>[2x]SMPITPQQALQRTIEHREIFHDEMVDLMRQIMRGEVSDAMVS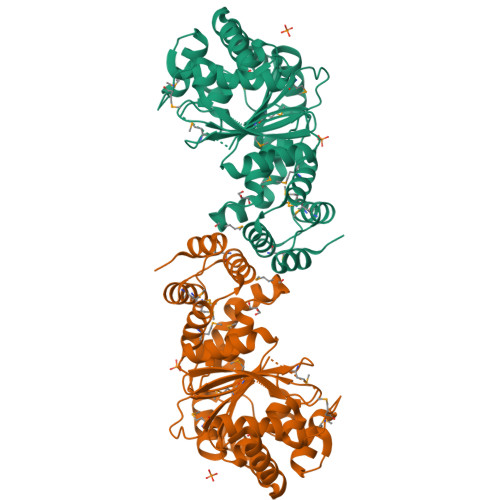AILTGLRVKKETIGEIAGAATVMREFSRRVEVTDRRHMVDIVGTGGDGSHTFNISTCAMFVAAAGGAKVAKHGNRSVSSKSGSADALEALGAVIELQPEQVAASLAQTGIGFMYAPVHHPAMKVVAPVRREMGVRTIFNILGPLTNPAGSPNILMGVFHPDLVGIQARVLQELGAERALVVWGRDGMDELSLGAGTLVGELRDGQVHEYEVHPEDFGIAMSASRNLKVADAAESRAMLLQVLDNVPGPALDIVALNAGAALYVAGVADSIADGIVRARQVLADGSARACLDAYVAFTQQATAQG>HHHHHHASAPCDSGWTLINKGDPFCAKQQSVTGTNFATSMTQCLNNGGKLCDLQEAVGMCQTGFIPSNTT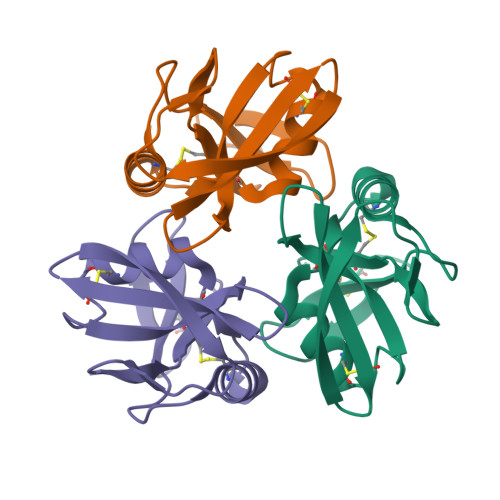LWISQLADNSSAHVINCTSGSWSAGFYGFGVTVDGSNPILPYCCKGRR[3x]>MASRQLATSHTAASNVSVAGDDGIDAELWYACAGPQKALPPVGSVVAYLPQGHIEQVASFNNQELDAQIPRYNLPAVIPCMLNDIQLSADPDSDEVYATLTLCPMSEQHEDSSDCAEPPPPPKRKSRSFTKTLTVSDTSTHGGFSVPRRAADDCLPKLDMSLNPPNQELVAKDLHGNEWRFRHIFRGQPKRHLLTTGWSVFVSQKRLVAGDAVLFLRGENGQLRVGVRRAPRQQQLQPKVLTSPTMHIGVLAAAAHAATEKSRFSLIYN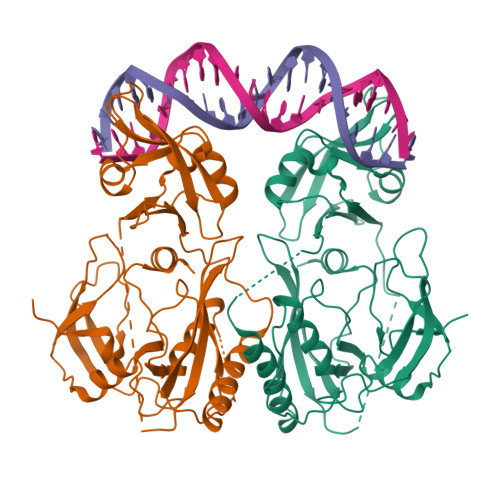PRSCPSEFVIPYSKYLKAVKSNFNVGQRFKMKFESEDPSDRRHTGTITGICDFDPARWPGSEWRSLQVNWDESSSSERQERVSPWEVEPGNSYSQSM[2x]>[6x]ASTLNAQIPELK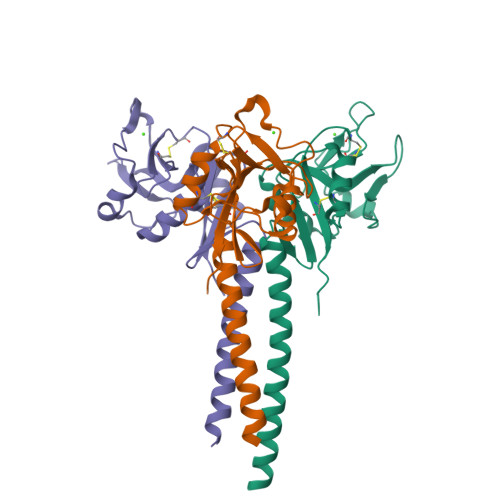SDLEKASALNTKIRALQGSLENMSKLLKRQNDILQVVSQGWKYFKGNFYYFSLIPKTWYSAEQFCVSRNSHLTSVTSESEQEFLYKTAGGLIYWIGLTKAGMEGDWSWVDDTPFNKVQSARFWIPGEPNNAGNNEHCGNIKAPSLQAWNDAPCDKTFLFICKRPYVPSEP>[9x]MTLLEVIIVLGIMGVVSAGVVTLAQRAIDSQNMTKAAQSLNSIQVALTQTYRGLGNYPATADATAASKLTSGLVSLGKISSDEAKNPF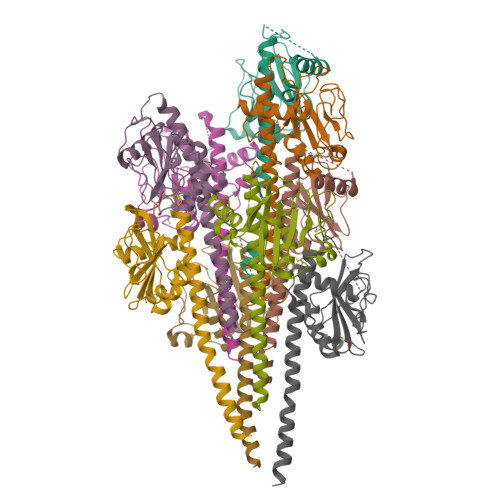IGTNMNIFSFPRNAAANKAFAISVDGLTQAQCKTLITSVGDMFPYIAIKAGGAVALADLGDFENSAAAAETGVGVIKSIAPASKNLDLTNITAVEKLCKGTAPFGVAFGNS>AQVINTFDGVADYLQTYHKLPDNYIAKSEAQALGWVASKGNLADVAPGKSIGGDIFSNREGKLPGKSGRTWREADINYTSGFRNSDRILYSSDWL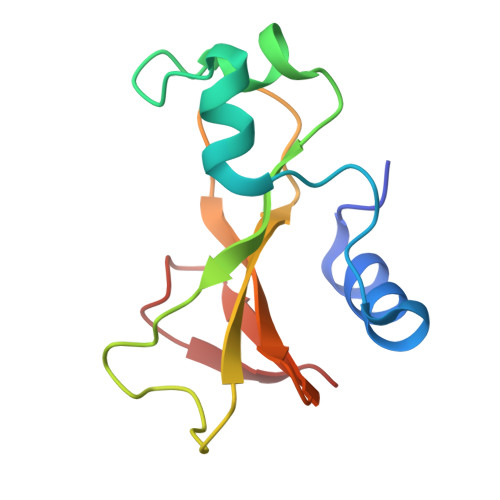IYKTTDHYQTFTKIR[3x]> MSQRPFYDGPMPTPRQKPFQSGSTPLHLTHRFMVWNSIGIIRCYNDEQDNAIDVEFHDTSIHHATHLSNTLNYTIADLSHEAILLACESTDELASKLHCLHFSSWDSSKEWIIDLPQNEDIEAICLGQGWAAAATSALLLRLFTIGGVQKEVFSLAGPVVSMAGHGEQLFIVYHRGTGFDGDQCLGVQLLELGKKKKQILHGDPLPLTRKSYLAWIGFSAEGTPCYVDSEGIVRMLNRGLGNTWTPICNTREHCKGKSDHYWVVGIHENPQQLRCIPCKGSRFPPTLPRPAVAILSFKLPYCQIATEKGQMEEQFWRSVIFHNHLDYLAKNGYEYEESTKNQATKEQQELLMKMLALSCKLEREFRCVEL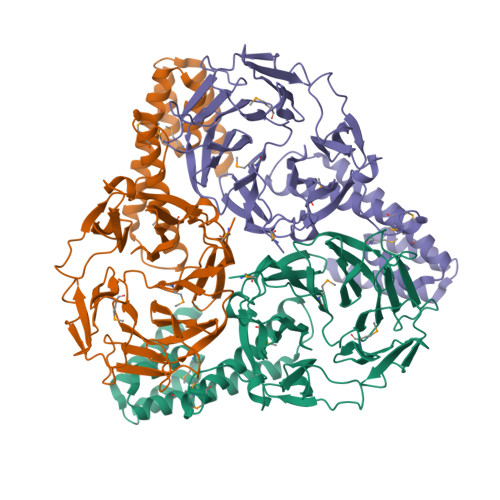ADLMTQNAVNLAIKYASRSRKLILAQKLSELAVEKAAELTATQVEEEEEEEDFRKKLNAGYSNTATHHHHHH>[2x]HHNKVRTCWNEGRPALAGWLQLPGTLHAEALARLDYDAVVIDMQHSPIDFGQVAPMLIAIELGGAEPFVRTQVNDPSDIMKLLDAGAYGIIAPMVNTRAEAQTLASALHYSPRGLRAFGPRRPSLRYGSGYLAQASETVVGLAMIETREALANIDEILSVDGIDGVFIGPTDLALDLGHAPLVDTEEA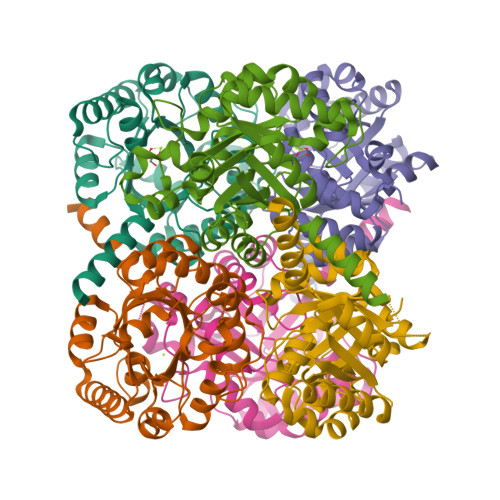EVVSAIAHVRERAHAAGKRVGIFCGSGGFARVKLAEGFDFVTAAPDLAMLSAAARQVIADARAL> GIDPFTMVSVDNTYQSLERELANDDPWRLDDNPFERERHTQLLRLSLSSGAVSNGLEIGCAAGAFTEKLAPHCKRLTVIDVMPRA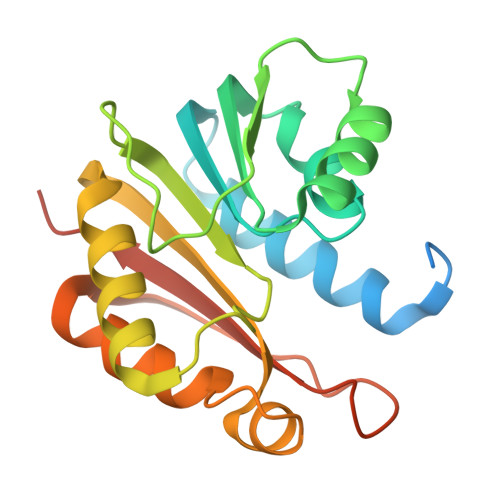IGRACQRTKRWSHISWAATDILQFSTAELFDLIVVAEVLYYLEDMTQMRTAIDNMVKMLAPGGHLVFGSARDATCRRWGHVAGAETVITILTEALTEVERVQCQGQSADEDCLLARFRNPERSSIRPDGRA>MKKRILAVAVTSMLLSASVFAQETVVPSRVGDLKFESDFPTQETMKNMLNEMDFQRATQAYLWGIPASSIMEWLNVSRNDFKFEEGQMGFFNTLKQKQGIITANFTTP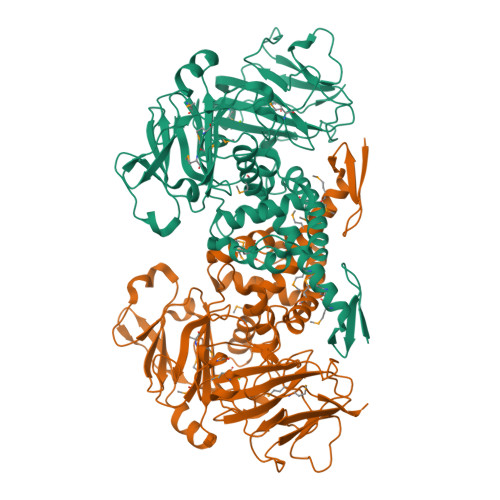YVIGTWNLEKTGPLIINLPEAKMAGMMLDVHQRVLSDLSLLGPDKGKGGKYLIVPPGEKYKDLNPKGYYVIRPKTNVVYGGIRILEPDVDRVVKQVVPNITTQPYADGKLGRKIPVAQVPEIDWTHIPKDGLEYWKTIHQIIQENPVEERDRFVMAQLKFLGIEKGKPFNPTEEQKKILLEASKVGRAMAQSNDYTKRFTQPYWKGTNWKDAISVSLDQRSENYDELDERAAWFYEAITVSRGMKSTIPGFGQRYLVTYQDSDGNWLSGEHTYKLHVPANVPASNFWSTTVYDENNRLMIINDAGSPDISSRKNLKVNSDGSIDVYYGPKPVKGYENNWVQTNPGEGWFTYFRFYGPTEKMFDKSWTMGDIELVK[4x]1-[3-(6-Methyl-2,3-dihydropyrazolo[5,1-b][1,3]oxazol-7-yl)indol-1-yl]ethanone | C16 H15 N3 O2 | 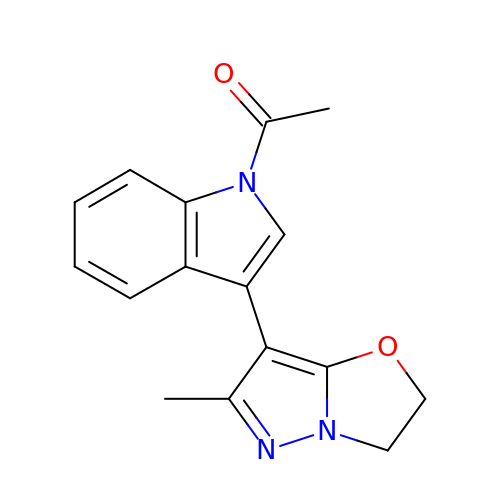RVHAVBXZRUCGCC-UHFFFAOYSA-N> MVSPTKMIIRSPLKETDTNLKHNNGIAASTTAAGHLNVFSNDNNCNNNNTTESFPKKRSLERLELQQQQHLHEKKRARIERARSIEGAVQVSKGTGLKNVEPRVTPKELLEWQTNWKKIMKRDSRIYFDITDDVEMNTYNKSKMDKRRDLLKRGFLTLGAQIT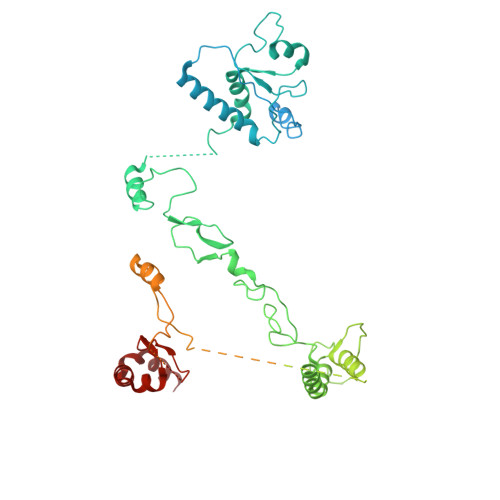QFFDTTVTIVITRRSVENIYLLKDTDILSRAKKNYMKVWSYEKAARFLKNLDVDLDHLSKTKSASLAAPTLSNLLHNEKLYGPTDRDPRTKRDDIHYFKYPHVYLYDLWQTWAPIITLEWKPQELTNLDELPYPILKIGSFGRCPFIGDRNYDESSYKRVVKRYSRDKANKKYALQLRALFQYHADTLLNTSSVNDQTKNLIFIPHTCNDSTKSFKKWMQEKAKNFEKTELKKTDDSAVQDVRNEHADQTDEKNSILLNETETKEPPLKEEKENKQSIAEESNKYPQRKELAATPKLNHPVLATFARQETEEVPDDLCTLKTKSRQAFEIKASGAHQSNDVATSFGNGLGPTRASVMSKNMKSLSRLMVDRKLGVKQTNGNNKNYTATIATTAETSKENRHRLDFNALKKDEAPSKETGKDSAVHLETNRKPQNFPKVATKSVSADSKVHNDIKITTTESPTASKKSTSTNVTLHFNAQTAQTAQPVKKETVKNSGYCENCRVKYESLEQHIVSEKHLSFAENDLNFEAIDSLIENLRFQI> GGUAXUGCGGUAC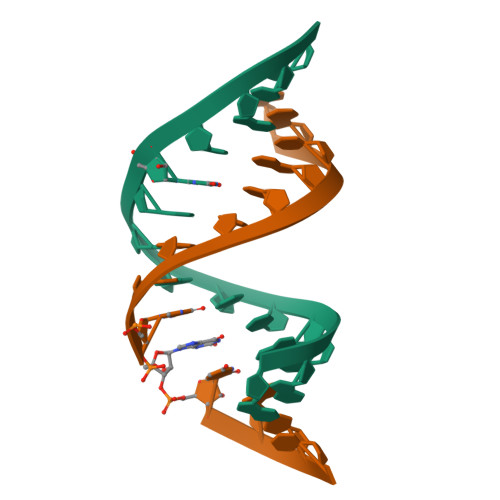C;> GGUACUGCGXUACC>MGSSHHHHHHSGLVPRGSHMATPPKRSSPSFSASSEGTRIKKISIEGNIAAGKSTFVNILKQLSEDWEVVPEPVARWSNVQSTQDEFEELTMSQKNGGNVLQMMYEKPERWSFTFQTYACLSRIRA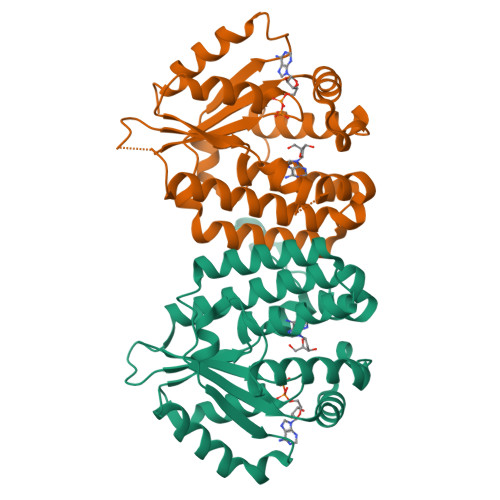QLASLNGKLKDAEKPVLFFERSVYSDRYIFASNLYESESMNETEWTIYQDWHDWMNNQFGQSLELDGIIYLQATPETCLHRIYLRGRNEEQGIPLEYLEKLHYKHESWLLHRTLKTNFDYLQEVPILTLDVNEDFKDKYASLVEKVKEFLSTL[2x]> GRKKIQITRIMDERNRQVTFTKRKFGLMKKAYELSVLCDCEIALIIFNSSNKLFQYASTDMDKVLLKYT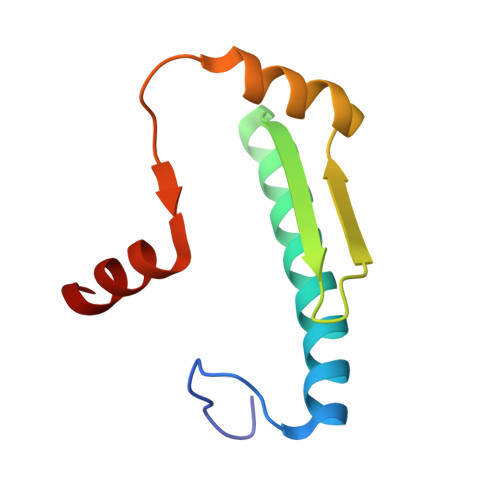EYNEPHESRTNSDIVEALNKK>[2x]MEPVIIGALILDVHAKPSTTPISGTTVPGQVLFAPGGVARNVADCIFKLGITPFMIGTLGLDGPANVLLKEWKLSMKGI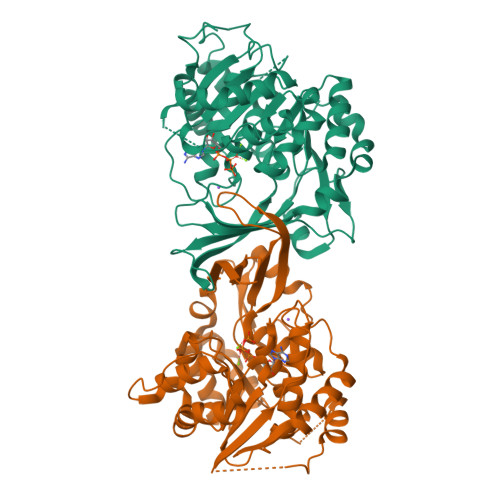LRREDISTPIVSLVYDTNGEVAAGVAGVDAVENFLTPEWIQRFEYNISSARLLMVDANLSSLALEASCKLAAESSVPVWFEPVSVTKSQRIASIAKYVTIVSPNQDELIAMANALCAKNLFHPFRSDENKLSIEDMFRALKPAILVLLKNGVKVVIVTLGSNGALLCSKGNPKKALNIDRKFLRSGEVFKRVQSVCSPNRFSELGSNRSPSLFAMHFPTIPAKVKKLTGAGDCLVGGTVASLSDGLDLIQSLAVGIASAKAAVESDDNVPPEFKLDLISGDAELVYNGAKMLMVHQSML>[4x]QKKKVTVEDLFSEDFKIHDPEAKWISDTEFIYREQKGTVRLWNVETNTSTVLIEGKKIESLRAIRYEISPDREYALFSYNVEPIYQHSYTGYYVLSKIPHGDPQSLDPPEVSNAKLQYAGWGPKGQQLIFIFENNIYYCAHVGKQAIRVVSTGKEGVIYNGLSDWLYEEEILKTHIAHWWSPDGTRLAYAAINDSRVPIMELPTYTGSIYPTVKPYHYPKAGSENPSISLHVI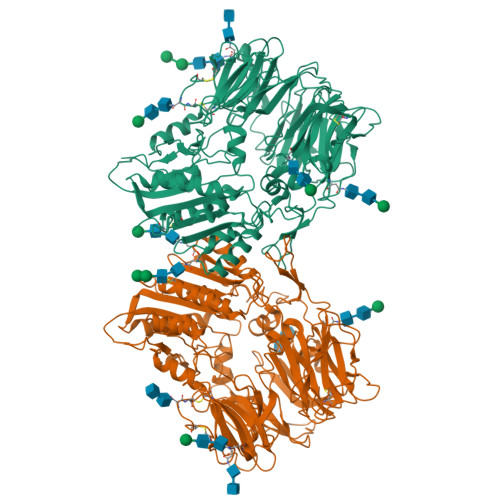GLNGPTHDLEMMPPDDPRMREYYITMVKWATSTKVAVTWLNRAQNVSILTLCDATTGVCTKKHEDESEAWLHRQNEEPVFSKDGRKFFFIRAIPQGGRGKFYHITVSSSQPNSSNDNIQSITSGDWDVTKILAYDEKGNKIYFLSTEDLPRRRQLYSANTVGNFNRQCLSCDLVENCTYFSASFSHSMDFFLLKCEGPGVPMVTVHNTTDKKKMFDLETNEHVKKAINDRQMPKVEYRDIEIDDYNLPMQILKPATFTDTTHYPLLLVVDGTPGSQSVAEKFEVSWETVMVSSHGAVVVKCDGRGSGFQGTKLLHEVRRRLGLLEEKDQMEAVRTMLKEQYIDRTRVAVFGKDYGGYLSTYILPAKGENQGQTFTCGSALSPITDFKLYASAFSERYLGLHGLDNRAYEMTKVAHRVSALEEQQFLIIHPTADEKIHFQHTAELITQLIRGKANYSLQIYPDESHYFTSSSLKQHLYRSIINFFVECFRI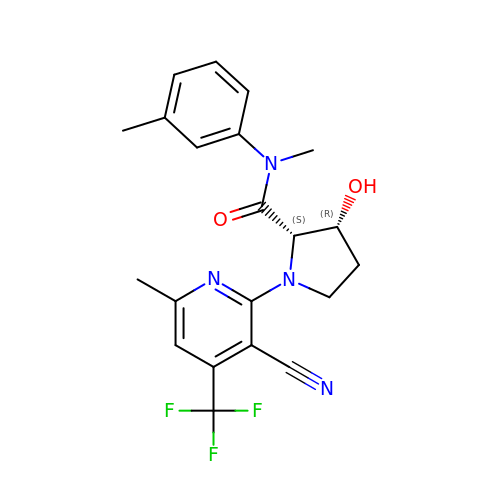(2~{S},3~{R})-1-[3-cyano-6-methyl-4-(trifluoromethyl)pyridin-2-yl]-~{N}-methyl-~{N}-(3-methylphenyl)-3-oxidanyl-pyrrolidine-2-carboxamide | C21 H21 F3 N4 O2 | YHMDHAMZFMNMTF-MSOLQXFVSA-N> GGCUUAUCAAGAGAGGGAGAGCGACUGGCGCGAAGACCCCCGGCAACCAGAAAUGGUGCCAAUUCCUGCAGCGGAAACGUUGAAAGA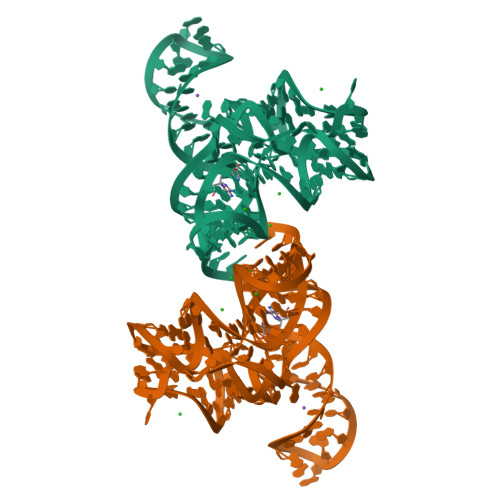UGAGCCA> GPLGSEEGLFSQKSFLVLGFSNENESNIANIIKENAGKIMSLLSRTVADYAVVPLLGCEVEA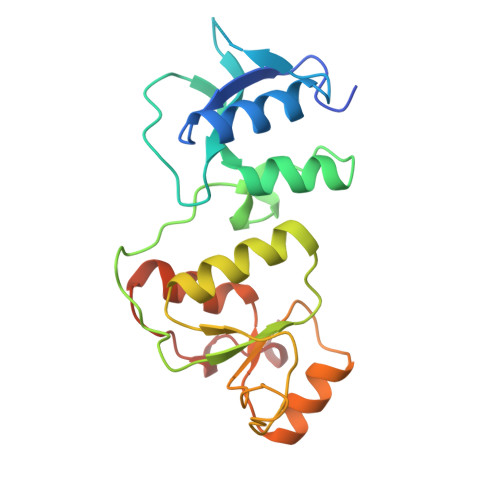TVGEVVTNTWLVTCIDYQTLFDPKSNPLFTPVPVMTGMTPLEDCVISFSQCAGAEKESLTFLANLLGASVQEYFVRKSNAKKGMFASTHLILKERGGSKYEAAKKWNLPAVTIAWLLETARTGKRADESHFLIENSTKEER> EEVIVEKTKQTVASISSGPKHTQKVPILTANETGATMPVLPSDSIETRTTYMHFNGSETDVECFLGRAACVHVTEIQNKDATGIDNHREAKLFNDWKINLSSLVQLRKKLELFTYVRFDSEYTILATASQPDSANYSSNLVVQAMYVPPGAPNPKEWDDYTWQSASNPSVFFKVGDT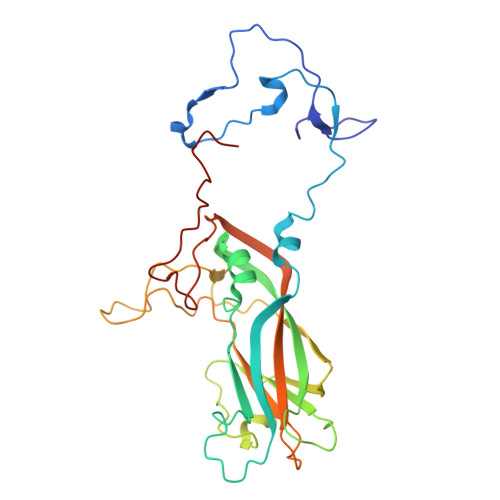SRFSVPYVGLASAYNCFYDGYSHDDAETQYGITVLNHMGSMAFRIVNEHDEHKTLVKIRVYHRAKHVEAWIPRAPRALPYTSIGRTNYPKNTEPVIKKRKGDIKSY ACETYL COENZYME *A | C23 H38 N7 O17 P3 S | 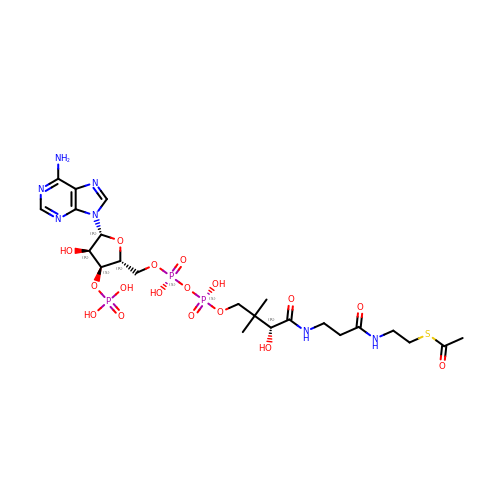ZSLZBFCDCINBPY-ZSJPKINUSA-N(2S,4S)-N-[(3R,5R)-1-cyclopropylcarbonyl-5-[[[4-[2-[4-[(1S)-2-methoxy-1-oxidanyl-ethyl]phenyl]ethynyl]phenyl]carbonylamino]methyl]pyrrolidin-3-yl]-4-fluoranyl-pyrrolidine-2-carboxamide 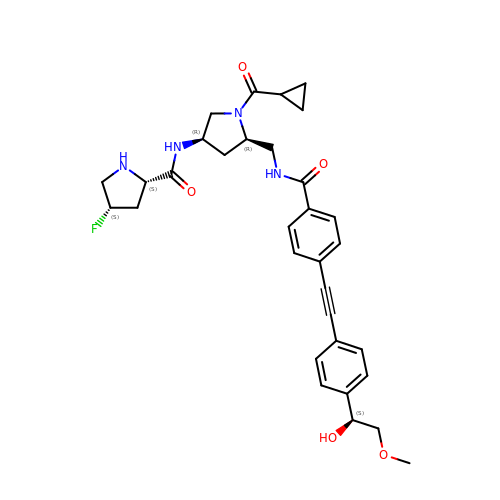| C32 H37 F N4 O5 | IKKZQZOORIUDON-MLZSXWJDSA-N>MSYVSAEHDRMLAAMILPCVVVAVDLAAARVRVRSGDWTSGWLRWHSLAAGKVRHWRAPSIGEQGVLLSPSGGVSMGTFIPGLYGDAGTAPDNSASSETWRFDDGASLSYDWAAHRYRVELPSGTVEV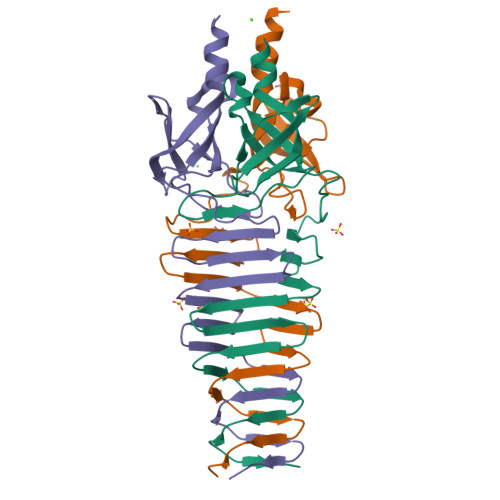RVGASEVRVSDGAVSLKAPKISLEGPVEIAGTLTVSGDILGGGSIIDTAGNSNHHTH[18x]>GSSSGRQGGVHELSAFEQLVVELVRHDDSWPFLKLVSKIQVPDYYDIIKKPIALNIIREKVNKCEYKLASEFIDDIELMFSNCFEYNPRNTS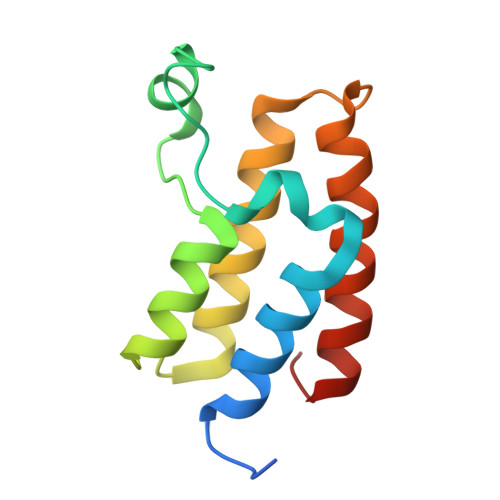EAKAGTRLQAFFHIQAQKLGLHVT[4x]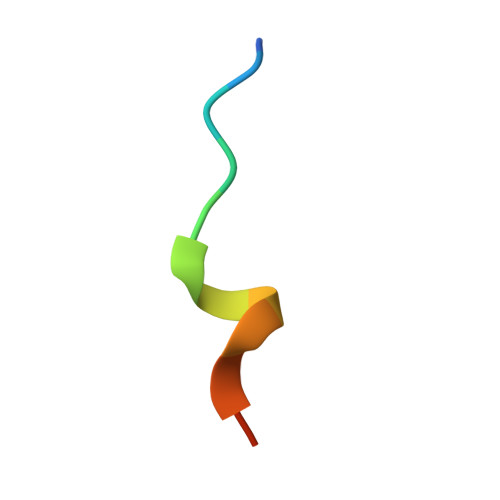> SPQKLIDGFLKHE> MDVNVNIDTNAEKQAISPYIYGTNQDFSNAKVTARRIGGNRSTGYNWENNDSNAGTDWKNESDNYWLTLYDVPKEKYNEPASVYTAFHDKSLAMGVPYSLVTLQAGGYVAADQSGPLANTDVAPSSKWKKVEFNKNGPLSLTPDTTDGSVYMDEFVNYLVNKYGSASGSKGIKGYSLDNEPSLWPSTHPLIHPDKTKCSEVLDKDTQLAQVVKKIDPAAETFGPALFGFSAFNDFNSSPDWSSVKGNYQWFIDYYLDNMKKNSDAAGKRLLDALDLHWYPEAKGGGQRVTTSDTSNVDCNKARMQAPRSLWDSTYTEDSWIGQWCKWGLPLIPKVKSSIDKYYPGTKLSFSEYNYGGEDHISGGIAQADALGVFGKYGVYFATYWECNSDKNNYVQSAFNLYNNYDGNNS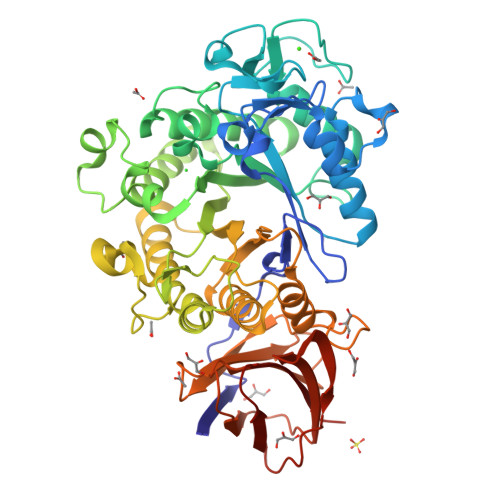KYGDTDVKCDTSDINNSSTYASVTSNDGNKMDIIVMNKNYTDSINFNFNVSSNKNYTSGQVWGFDSNSSNITKRDDVSSISGNKFTYKIPALTAVHIVLLEHHHHHH>MSLIWKRKITLEALNAMGEGNMVGFLDIRFEHIGDDTLEATMPVDSRTKQPFGLLHGGASVVLAESIGSVAGYLCTEGEQKVVGLEINANHVRSAREGRVRGVCKPLHLGSRHQVWQIEIFDEKGRLCCSSRLTTAIL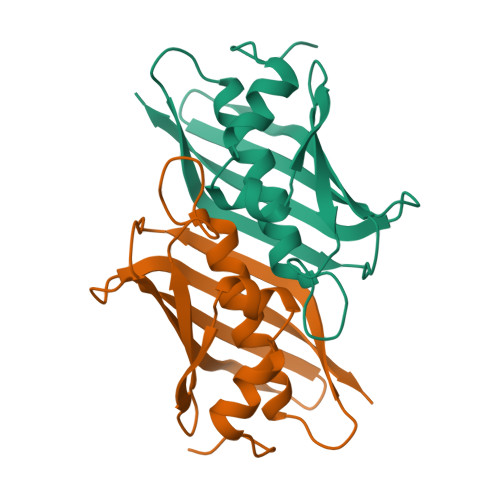EGGSHHHHHH[2x]> MKHHHHHHHMVSTLKPLKIGKHTIKFPIFQGGMGVGISWDELAGNVAKEGALGVISAVGTGYYKNMRFVERIVAKKPFEALNFYSKKALNEIFANARKICGNNPLGANILY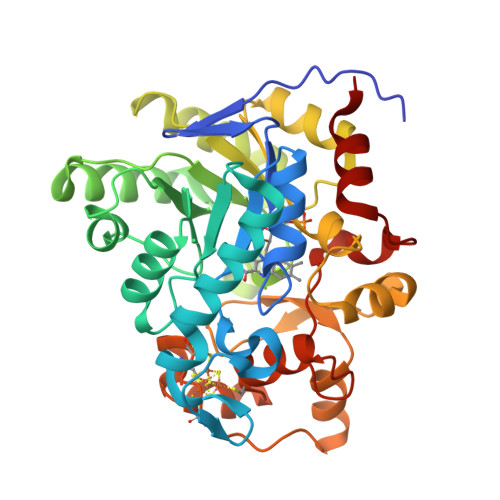AINDYGRVLRDSCEAGANIIITGAGLPTNMPEFAKDFSDVALIPIISSAKALKILCKRWSDRYKRIPDAFIVEGPLSGGHQGFKYEDCFKEEFRLENLVPKVVEASKEWGNIPIIAAGGIWDRKDIDTMLSLGASGVQMATRFLGTKECDAKVYADLLPTLKKEDILLIKSPVGYPARAINTGVIKRIEEGNAPKIACVSNCVAPCNRGEEAKKVGYCIADGLGRSYLGNREEGLYFTGANGYRVDKIISVHELIKELTEG>MVSDYVPDAGHLVWLNFTPQAGHEQGGRRPALVLSPAAYNGVTGLMQACPVTSRAKGYPFEVTLPAHLGVSGVVLADHCRSLDWRSRRAEQLAEAPAD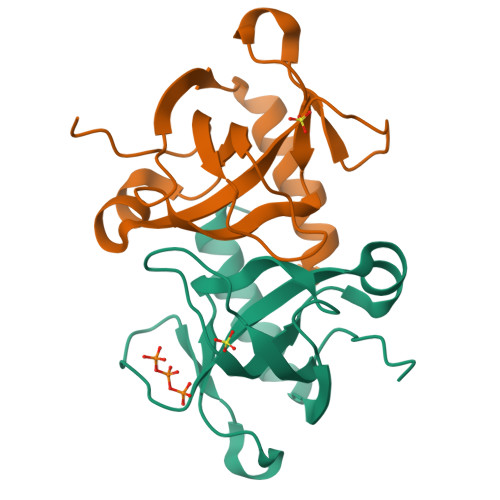VLAEVRGKLGSLLGMSEKA[2x]>[4x]G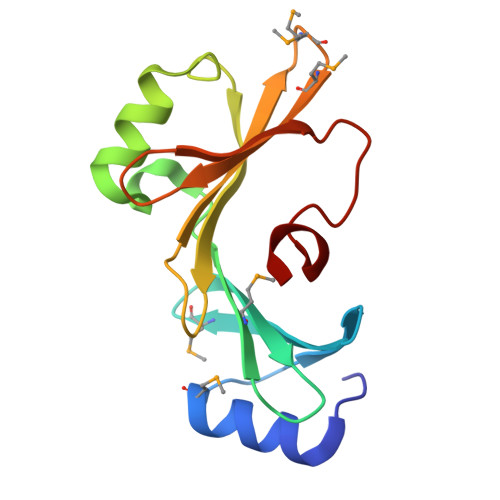GYAPDSVQIALKKMYPTAAGIAWSQDKAYYVADFVMNGFDTRVWFTPDAEWVMKQTDWETLDEVPAAVFNAFAASEFSDGVVQNVTWVQFPEWQPIVAIQVGKPNMQMKYQILFTPKGEVLRQQNITNAYNTLGASTFL> NDLLSIPVNSIYEEKYDKRWLTVFGFSHDKTDLIVDELSKYGNIIEIEYPQQPNCNWIYLKFESEY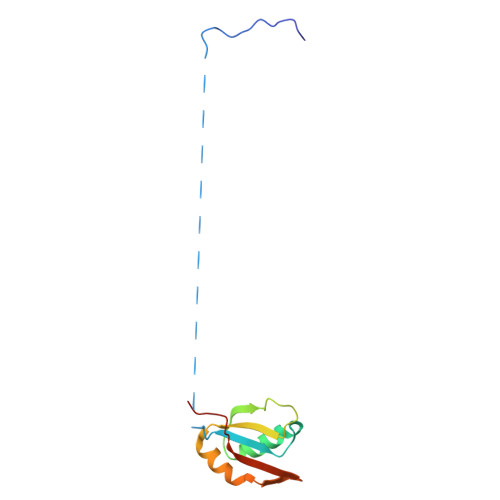SSIDLLKKNGLILGNCMIGIVPCKEKIRN The most frequent PTM reaction catalyzed by FIC enzymes is the addition of AMP using ATP as a cofactor, coined AMPylation or adenylylation. Enterococcus faecalis FIC belongs to class III FIC proteins, which are comprised of a single FIC domain and carry an autoinhibitory glutamate in their C-terminal α-helix. We discover that EfFIC has both AMPylation and deAMPylation activities borne by the same active site. Furthermore, the conserved glutamate implements a Ca2+-controlled metal switch that tunes the balance between these activities without conformational change.

We determined crystal structures of unbound, phosphate-bound, AMP-bound, and ATPγS-bound wild-type EfFIC (EfFICWT) and of unbound and sulfate-bound EfFIC carrying a mutation of the catalytic histidine into an alanine (EfFICH111A). Two crystal structures were obtained by co-crystallization with a non-hydrolyzable ATP analog (ATPγS), for which well-defined electron density was observed for the ADP moiety. E190 has the same conformation as in other glutamate-bearing FIC protein structures and is stabilized by a salt bridge with Arg122 and, when present, by interactions with the nucleotide cofactor. Based on the observations that the α- and β-phosphates of ATP bind with canonical positions to wild-type EfFIC and that AMPylation is potentiated by mutation of the conserved glutamate in various FIC proteins, we propose that the primary role of this glutamate in AMPylation is to mitigate the efficiency of this reaction in the presence of Mg2+, rather than to fully repress it, possibly in order to match AMPylation and deAMPylation efficiencies.

>[6x]MHHHHHHMLENKLGIINQLELNRVEERVSKENAKRLYDSGDIDRIEVGTFKGLSYIHNYLFEDIYEFAGKVRSQNISKGNFRFAPVMYLEIALEHIDKMPQRNLDEIVAKYVEMNIAHPFREGNGRATRIWLDLILKKELKRVVDWNLINKEDYLSAMERSPVKDLEIKYLISNALTDKINDREIFMKGIDISYYYEGYTEYNVDEL> MSEIGTGFPFDPHYVEVLGERMHYVDVGPRDGTPVLFLHGNPTSSYLWRNIIPHVAPSHRCIAPDLIGMGKSDKPDLDYFFDDHVRYLDAFIEAL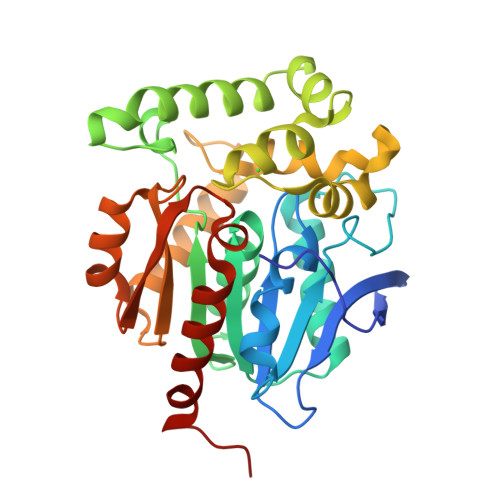GLEEVVLVIHDWGSALGFHWAKRNPERVKGIACMEFIRPIPTWDEFHHTEVAEEQDHAEAARETFQAFRTADVGRELIIDQNAFIERVLPGGVVRPLTEVEMDHYREPFLKPVDREPLWRFPNELPIAGEPANIVALVEAYMNWLHQSPVPKLLFWGTPGALIPPAEAARLAESLPNCKTVDIGPGLHYLQEDNPDLIGSEIARWLPALEHHHHHH> MLSQIAICIWVESTAILQDCQRALSADRYQLQVCESGEMLLEYAQTHR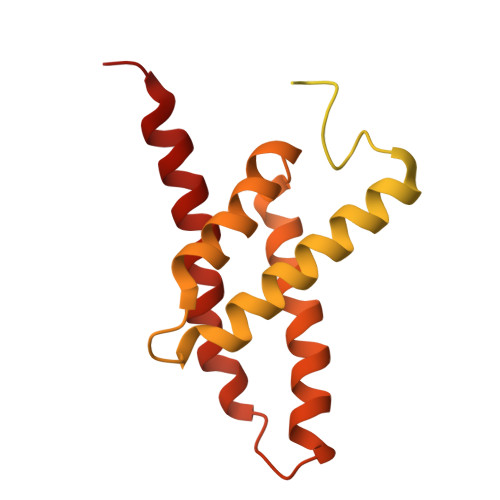DQIDCLILVAANPSFRAVVQQLCFEGVVVPAIVVGDRDSEDPDEPAKEQLYHSAELHLGIHQLEQLPYQVDAALAEFLRLAPVETMADHIMLMGANHDPELSSQQRDLAQRLQERLGYLGVYYKRDPDRFLRNLPAYESQKLHQAMQTSYREIVLSYFSPNSNLNQSIDNFVNMAFFADVPVTKVVEIHMELMDEFAKKLRVEGRSEDILLDYRLTLIDVIAHLCEMYRRSIPRET>MGTQTLSQLENSGAFIERHIGPDAAQQQEMLNAVGAQSLNALTGQIVPKDIQLATPPQVGAPATEYAALAELKAIASRNKRFTSYIGMGYTAVQLPPVILRNMLENPGWYTAYTPYQPEVSQGRLEALLNFQQVTLDLTGLDMASASLLDEATAAAEAMAMAKRVSKLKNANRFFVASDVHPQTLDVVRTRAETFGFEVIVDDAQKVLDHQDVFGVLLQQVGTTGEIHDYTALISELKSRKIVVSVAADIMALVLLTAPGKQGADIVFGSAQRFGVPMGYGGPHAAFFAAKDEYKRSMPGRIIGVSKDAAGNTALRMAMQTREQHIRREKANSNICTSQVLLANIASLYAVYHGPVGLKRIANRIHRLTDILAAGLQQKGLKLRHAHYFDTLCVEVADKAGVLTRAEAAEINLRSDILNAVGITLDETTTRENVMQLFNVLLGDNHGLDIDTLDKDVAHDSRSIQPAMLRDDEILTHPVFNRYHSETEMMRYMHSLERKDLALNQAMIPLGSCTMKLNAAAEMIPITWPEFAELHPFCPPEQAEGYQQMIAQLADWLVKLTGYDAVCMQPNSGAQGEYAGLLAIRHYHESRNEGHRDICLIPASAHGTNPASAHMAGMQVVVVACDKNGNIDLTDLRAKAEQAGDNLSCIMVTYPSTHGVYEETIREVCEVVHQFGGQVYLDGANMNAQVGITSPGFIGADVSHLNLHKTFCIPHGGGGPGMGPIGVKAHLAPFVPGHSVVQIEGMLTRQGAVSAAPFGSASILPISWMYIRMMGAEGLKKASQVAILNANYIASRLQDAFPVLYTGRDGRVAHECILDIRPLKEETGISELDIAKRLIDYGFHAPTMSFPVAGTLMVEPTESESKVELDRFIDAMLAIRAEIDQVKAGVWPLEDNPLVNAPHIQSELVAEWAHPYSREVAVFPAGVADKYWPTVKR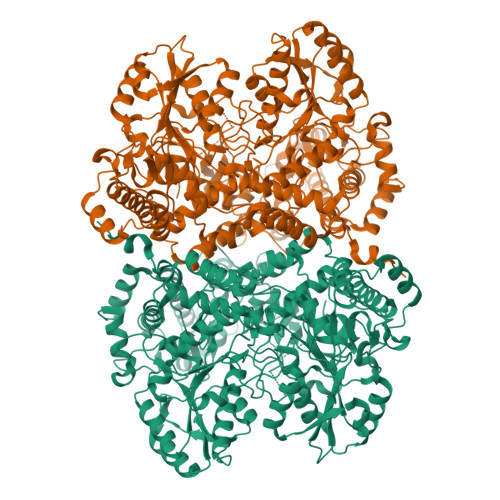LDDVYGDRNLFCSCVPISEYQLEHHHHHH[2x]2'-deoxy-5-ethynyluridine | C11 H12 N2 O5 | 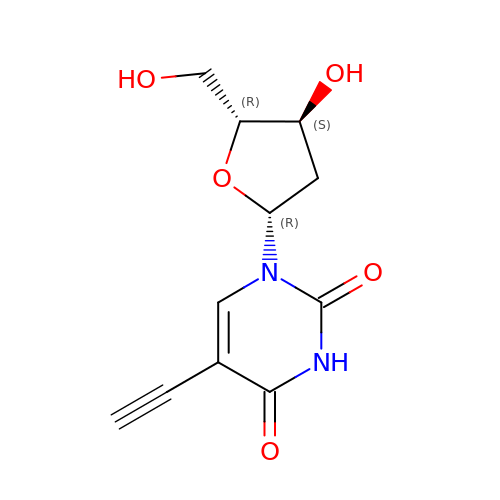CDEURGJCGCHYFH-DJLDLDEBSA-N> MQDNSRYTHFLTQHYDAKPQGRDDRYCESIMRRRGLTSPCKDINTFIHGNKRSIKAICENKNGNPHRENLRISKSSFQVTTCKLHGGSPWPPCQYRATAGFRNVVVACENGLPVHLDQSIFCRP

Angiogenin (ANG), a 14-kDa basic protein is an angiogenic ribonuclease and member of the bovine pancreatic ribonuclease (RNase A) family (also known as RNase 5). Like RNase A, ANG cleaves preferentially on the 3′ side of pyrimidines and follows a transphosphorylation/hydrolysis mechanism. In addition, the crystal structure of human ANG has revealed that it has an RNase A fold and the catalytic triad (residues H13, K40 and H114) is conserved. The enzymatic activity of ANG is several orders of magnitude lower than that of RNase A towards conventional RNase substrates, but essential for its angiogenic effect.

An important structural feature of ANG is that a part of the active site (i.e., the C-terminal region of the molecule) is obstructed by residue Q117 (part of the pyrimidine recognition site). It has been postulated that movement of Q117 and adjacent residues is required for substrate binding and catalysis. Mutational studies on C-terminal segment of ANG have also shown that shorter side-chain residues or deletion of residues affects the catalytic activity and previous structural studies have revealed that the segment containing residues 117–123 in the wild-type is highly mobile. In the 3D structure of native ANG, R121 forms part of a peripheral sub-site for binding polynucleotide substrates at the C-terminal region’s closed conformation. The ALS associated variant R121C has significantly higher RNase activity (131%) as compared with wild-type ANG. In the crystal structure of the variant, the smaller side-chain of cysteine appears to provide more flexibility for the C-terminal end of the molecule by destabilizing the closed conformation thus providing better access to substrates which would explain the enhanced RNase activity. Similar observations have been reported previously for the R121H ALS implicated variant8.4-{3-[(E)-2-cyanoethenyl]-5-fluorophenoxy}-3-[2-(2,4-dioxo-3,4-dihydropyrimidin-1(2H)-yl)ethoxy]phenyl 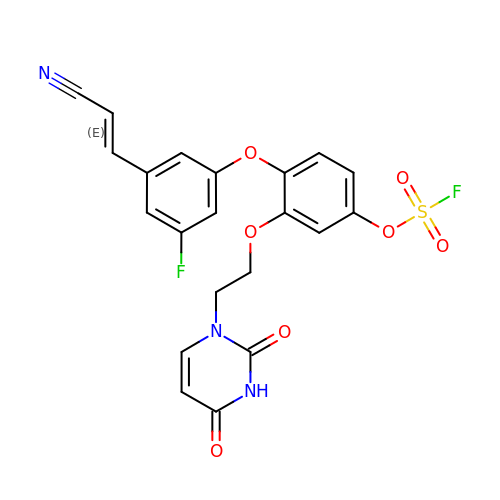sulfurofluoridate | C21 H15 F2 N3 O7 S | HGGIZBJCOFSILC-OWOJBTEDSA-N>MLIIETLPLLRQQIRRLRMEGKRVALVPTMGNLHDGHMKLVDEAKARADVVVVSIFVNPMQFDRPEDLARYP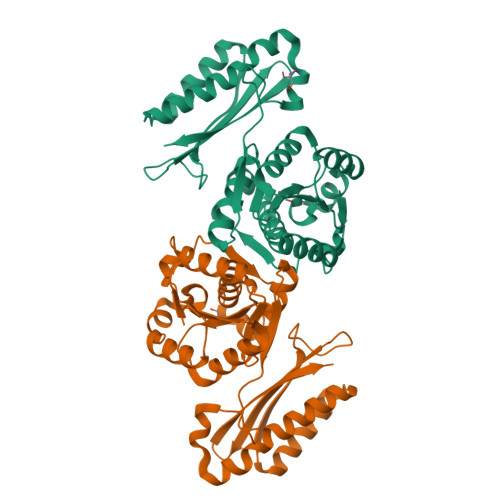RTLQEDCEKLNKRKVDLVFAPSVKEIYPNGTETHTYVDVPGLSTMLEGASRPGHFRGVSTIVSKLFNLVQPDIACFGEKDFQQLALIRKMVADMGFDIEIVGVPIMRAKDGLALSSRNGYLTAEQRKIAPGLYKVLSSIADKLQAGERDLDEIITIAGQELNEKGFRADDIQIRDADTLLEVSETSKRAVILVAAWLGDARLIDNKMVELA[2x]> MKFGQQLRSSIIREYQWHYIDYDGLKADLKRASGPLVASSDPTKPPRREWTEDDESRFVSKLEAELDKVHAKQQVKAMEISRRIAVSEREVQDVVGRLQDRGPGQEGPSEEEFMLLEEDLSDIIADVHDLAKFVQVNYTGFYKIIKKHDKMTGWRLKPVFDTRLKAKPFYKENYDASVVRLSKLYDLVRTRGNLEHHH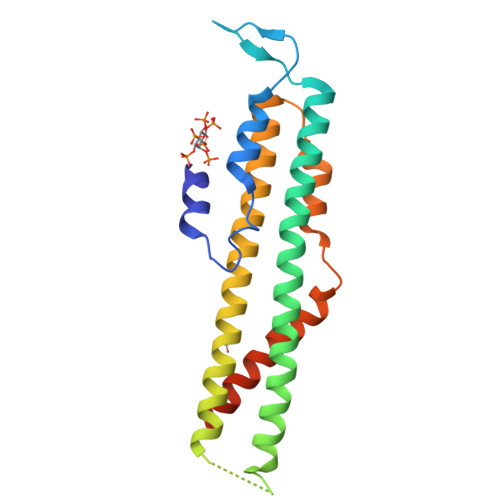HHH N-pentyl-L-alaninamide | C8 H18 N2 O | 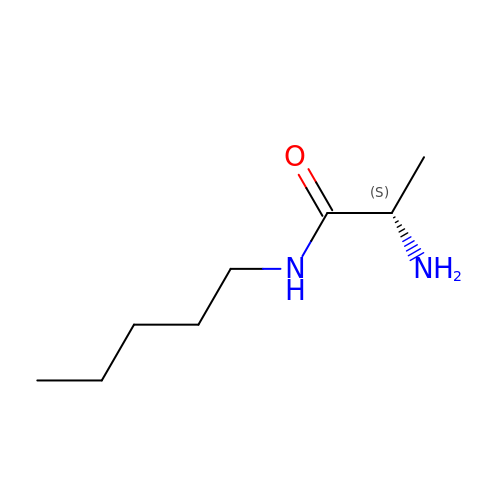XITIWNUYCSVDOK-ZETCQYMHSA-N> FTLYPYDTNYLIYTQTSDLNKEAIASYDWAENARKDEVKFQLSLAFPLWRGILGPNSVLGASYTQKSWWQLSNSEESSPFRETNYEPQLFLGFATDYRFAGWTLRDVEMGYNHDSNGRSDPTSRSWNRLYTRLMAENGNWLVEVKPWYVVGNT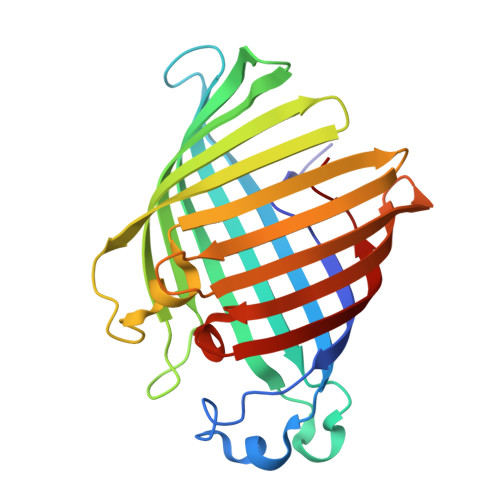DDNPDITKYMGYYQLKIGYHLGDAVLSAKGQYNWNTGYGGAELGLSYPITKHVRLYTQVYSGYGESLIDYNFNQTRVGVGVMLNDLF> AEPVQEELSVLAAIFCRPHEWEVLSRSETDGTVFRIHTKAEGFMDVDIPLELVFHLPVNYPSCL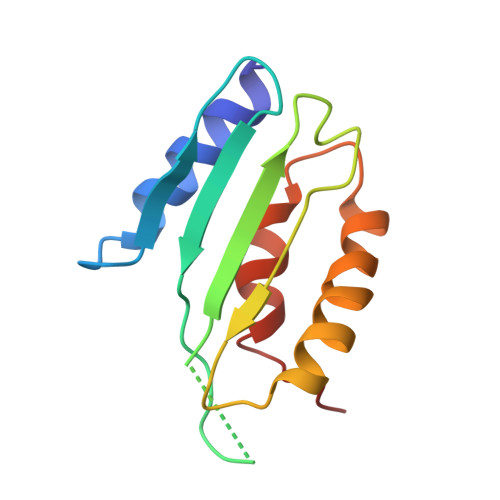PGISINSEQLTRAQCVTVKEKLLEQAESLLSEPMVHELVLWIQENLRHA>MSQHNEKNPHQHQSPLHDSSEAKPGMDSLAPEDGSHRPAAEPTPPGAQPTAPGSLKAPDTRNEKLNSLEDVRKGSENYALTTNQGVRIADDQNSLRAGSRGPTLLEDFILREKITHFDHERIPERIVHARGSAAHGYFQPYKSLSDITKADFLSDPNKITPVFVRFSTVQGGAGSADTVRDIRGFATKFYTEEGIFDLVGNNTPIFFIQDAHKFPDFVHAVKPEPHWAIPQGQSAHDTFWDYVSLQPETLHNVMWAMSDRGIPRSYRTMEGFGVHTFRLINAEGKATFVRFHWKPLAGKASLVWDEAQKLTGRDPDFHRRELWEAIEAGDFPEYELGFQLIPEEDEFKFDFDLLDPTKLIPEELVPVQRVGKMVLNRNPDNFFAENEQAAFHPGHIVPGLDFTNDPLLQGRLFSYTDTQISRLGGPNFHEIPINRPTCPYHNFQRDGMHRMGIDTNPANYEPNSINDNWPRETPPGPKRGGFESYQERVEGNKVRERSPSFGEYYSHPRLFWLSQTPFEQRHIVDGFSFELSKVVRPYIRERVVDQLAHIDLTLAQAVAKNLGIELTDDQLNITPPPDVNGLKKDPSLSLYAIPDGDVKGRVVAILLNDEVRSADLLAILKAL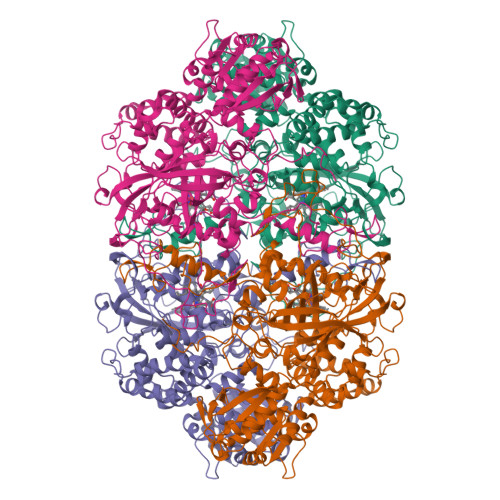KAKGVHAKLLYSRMGEVTADDGTVLPIAATFAGAPSLTVDAVIVPCGNIADIADNGDANYYLMEAYKHLKPIALAGDARKFKATIKIADQGEEGIVEADSADGSFMDELLTLMAAHRVWSRIPKIDKIPA[4x]> MAHHHHHHSL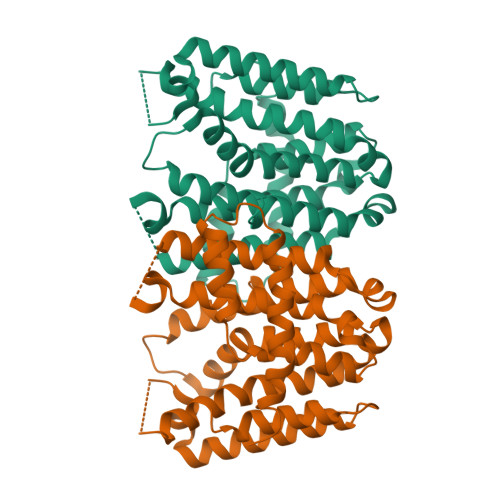EALSSYQQRNNQQLDQWLNRIPFQTLPLIEAMRYGLLLGGKRARPYLVYITGQMLGCELSDLDTPASAVECIHAYSLIHDDLPAMDDDELRRGKPTCHIQFDEATAILTGDALQTLAFTILAEGDLSAAGETQRVAMLQALAEASGAQGMCLGQALDLAAENRLISLEELETIHRNKTGALMRCAIRLGALAAGEKGRAMLPHLDRYAEAVGLAFQVQDDILDIISDTETLGKPQGSDQELNKSTYPALLGLEGAQQKAHTLLQEALLALEAIPYNTEHLEEFARYVVERKN> MVKQIES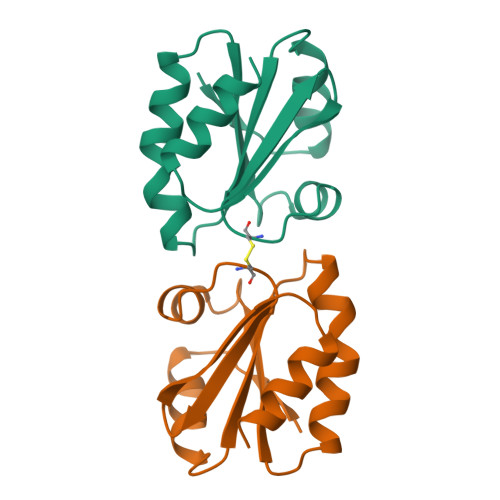KTAFQEALDAAGDKLVVVDFSATWSGPSKMIKPFFHSLSEKYSNVIFLEVDVDDCQDVASECEVKCMPTFQFFKKGQKVGEFSGANKEKLEATINELV> MPLDPRIKKLLESGFVVPIGKASVDEVRKIFRQLASAAPKAEVRKVEDIKIPGSETSINARVYFPKAKGPYGVLVYLHGGGFVIGDVESYDPLCRAITNACNCVVVSVDYRLAPEYKFPSAVIDSFDATNWIYNNLDKFDGEMGIAIAGDSAGGNLAAVVALLSKGKLDLKYQILIYPAVGFDSVSRSMIEYSDGFFLTREHIEWFGSQYLRSPADLLDFRFSPIIAQDLSGLPPALIITAEYDPLRDQGEAYANRLLQAGVPVTSVRFNNVIDGFLSFFPLIDQGKDAIG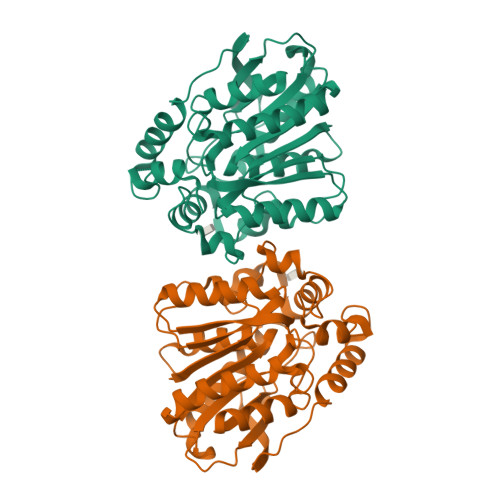LIGSVLRRTFYDKS L‐Asparaginases (ASNases) catalyze the hydrolysis of L‐Asn to L‐Asp and ammonia. In contrast, the chain of ASNase from Rhodospirillum rubrum, reported here and referred to as RrA, consists of only 172 amino acid residues. RrA is homologous to the N‐terminal domain of typical bacterial class 1 ASNases and exhibits millimolar affinity for L‐Asn. Crystal structures of the wild‐type RrA, both with and without bound L‐Asp, as well as structures of several RrA mutants, reveal topologically unique tetramers.

Another residue that was mutated in order to assess its importance for the catalytic activity was Lys19. This residue is highly conserved in scASNases but not in typical class 1 ASNases. We probed the importance of this residue by mutating it to L‐Ala, L‐Glu, and L‐Gln. In some cases, orthorhombic crystals with a doubled c axis were obtained, belonging to space group P212121. The a. u. for these crystals contained a complete tetramer. The kinetic data, even when reduced to approximate turnover numbers, demonstrate that Lys19 plays an important role during catalysis and its mutation reduces the rate of catalysis by two or more orders of magnitude. It appears that Lys19 may play a comparable function to Tyr21, each being responsible for both stabilizing the tetramer and for supporting proton transfer.

>[4x]HHHHHHENLYFQSMAVSPSPLRIFTAGGTIDADYRLEENGLVVGDPFVAEVLKTARLAGAVSIVALSRKDSLDFTEADREAIGRAVGQAVEDHILLTHGTDTMVETARYLGGLPELAGKTVVLSGAMVPGRVGGSDAAFNIGFACAAALMLAPGVYIAMHGKVFDPAKTRKNRGLGRFEPIDDQE> MLKGKDGVVKNASTGDSIGHLQSWALDTQRDEVSGWGMGDDAERAFTTVGRASGNFEVYLDPADPSDDLEPGDLVDLELYPGGESTGSGYRSVAGALILSTAESASKDGIPMLTVNWRTSGALPQK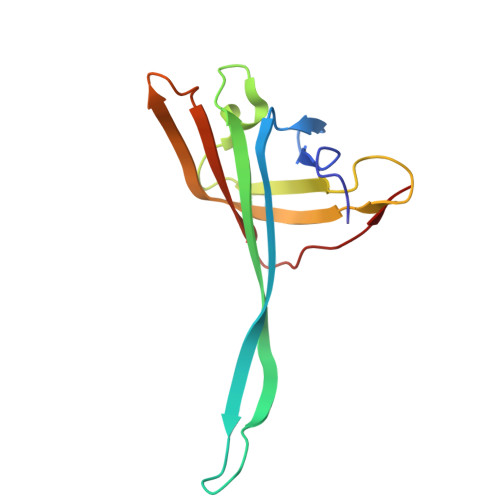ATVS>[4x]HHHHHHSSGLVPRGSHMASMSKVGINGFGRIGRLVLRRLLEVKSNIDVVAINDLTSPKILAYLLKHDSNYGPFPWSVDFTEDSLIVDGKSIAVYAEKEAKNIPWKAKGAEIIVECTGFYTSAEKSQAHLDAGAKKVLISAPAGEMKTIVYNVNDDTLDGNDTIVSVASSTTNCLAPMAKALHDSFGIEVGTMTTIHAYTGTQSLVDGPRGKDLRASRAAAENIIPHTTGAAKAIGLVIPELSG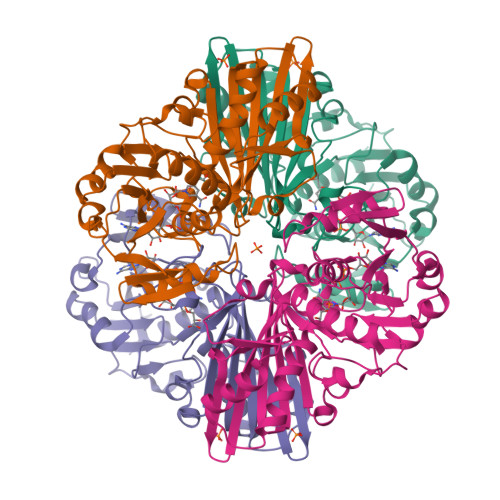KLKGHAQRVPVKTGSVTELVSILGKKVTAEEVNNALKQATTNNESFGYTDEEIVSSDIIGSHFGSVFDATQTEITAVGDLQLVKTVAWYDNEYGFVTQLIRTLEKFAKL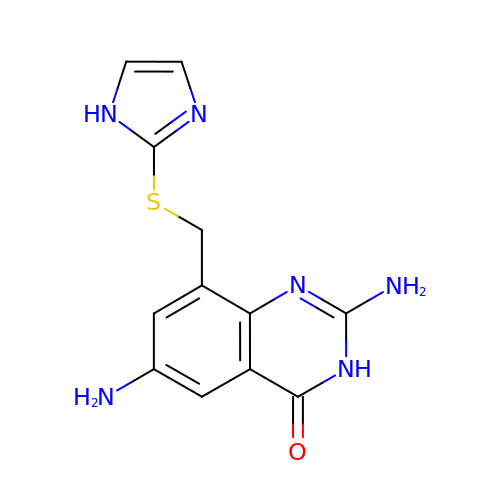2,6-DIAMINO-8-(1H-IMIDAZOL-2-YLSULFANYLMETHYL)-3H-QUINAZOLINE-4-ONE | C12 H12 N6 O S | CEWKWXPCQGWWBM-UHFFFAOYSA-N({3-hydroxy-2-oxo-4-[2-(phosphonooxy)ethyl]pyridin-1(2H)-yl}methyl)phosphonic 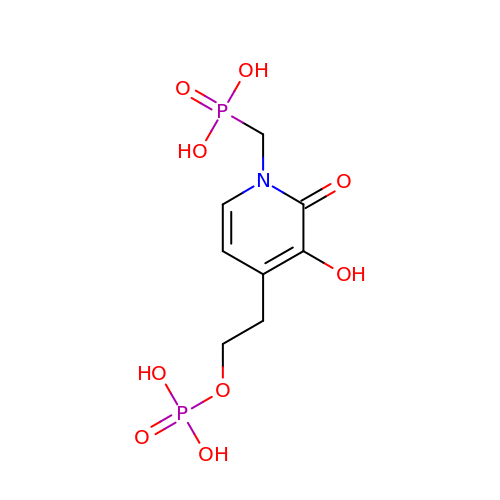acid | C8 H13 N O9 P2 | RMAJJEZWSTVCSS-UHFFFAOYSA-N> MSEKRSLPMVDVKIDDEDTPQLEKKIKRQSIDHGVGSEPVSTIEIIPSDSFRKYNSQGFKAKDTDLMGTQLESTFEQELSQMEHDMADQEEHDLSSFERKKLPTDFDPSLYDISFQQIDAEQSVLNGIKDENTSTVVRFFGVTSEGHSVLCNVTGFKNYLYVPAPNSSDANDQEQINKFVHYLNETFDHAIDSIEVVSKQSIWGYSGDTKLPFWKIYVTYPHMVNKLRTAFERGHLSFNSWFSNGTTTYDNIAYTLRLMVDCGIVGMSWITLPKGKYSMIEPNNRVSSCQLEVSINYRNLIAHPAEGDWSHTAPLRIMSFSISCAGRIGVFPEPEYDPVIQIANVVSIAGAKKPFIRNVFTLNTCSPITGSMIFSHATEEEMLSNWRNFIIKVDPDVIIGYNTTNFDIPYLLNRAKALKVNDFPYFGRLKTVKQEIKESVFSSKAYGTRETKNVNIDGRLQLDLLQFIQREYKLRSYTLNAVS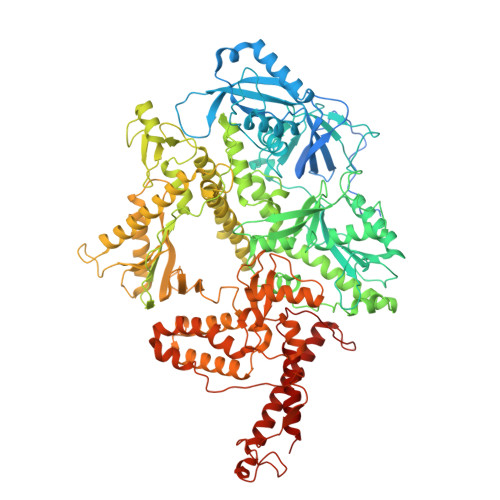AHFLGEQKEDVHYSIISDLQNGDSETRRRLAVYCLKDAYLPLRLMEKLMALVNYTEMARVTGVPFSYLLARGQQIKVVSQLFRKCLEIDTVIPNMQSQASDDQYEGATVIEPIRGYYDVPIATLDFNSLYPSIMMAHNLCYTTLCNKATVERLNLKIDEDYVITPNGDYFVTTKRRRGILPIILDELISARKRAKKDLRDEKDPFKRDVLNGRQLALKISANSVYGFTGATVGKLPCLAISSSVTAYGRTMILKTKTAVQEKYCIKNGYKHDAVVVYGDTDSVMVKFGTTDLKEAMDLGTEAAKYVSTLFKHPINLEFEKAYFPYLLINKKRYAGLFWTNPDKFDKLDQKGLASVRRDSCSLVSIVMNKVLKKILIERNVDGALAFVRETINDILHNRVDISKLIISKTLAPNYTNPQPHAVLAERMKRREGVGPNVGDRVDYVIIGGNDKLYNRAEDPLFVLENNIQVDSRYYLTNQLQNPIISIVAPIIGDKQANGMFVVKSIKINTGSQKGGLMSFIKKVEACKSCKGPLRKGEGPLCSNCLARSGELYIKALYDVRDLEEKYSRLWTQCQRCAGNLHSEVLCSNKNCDIFYMRVKVKKELQEKVEQLSKW> MDVQLPYNVKIEAFEGPLDLLLHLINRYEIDIYDI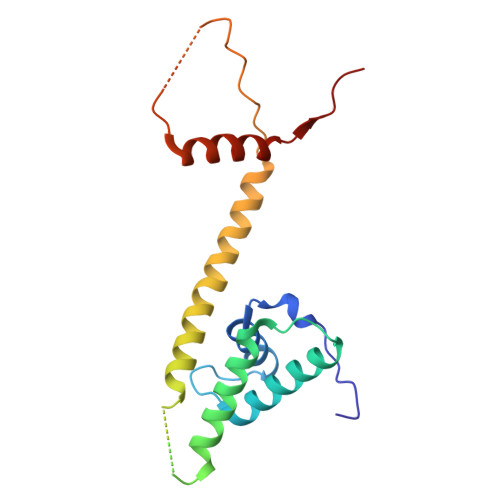PVAQITEQYMAYIHAMQELELDIASEYLVMAATLLAIKSKMLLPPSNEEAVDGDIEWGDDGDPREELTQRLLEYKKFKEAARELKRREEERALLFTKPPSDLSAYADEKKAAPLDVNVYDMLGALSKLLRRKKLQKPMR> MERLVWDKLTLLGFLEKNHIPQKLYYNLSSQDKELSAEIQSNVTYYTLRDANNTLIQALIPISQDLQIHIYKKGEDYFLDFIPIIFTRKEKTLLLSLQTSPYQDIIKATNDPLLANQLMNAYKKSVPFKRLVKNDKIAIV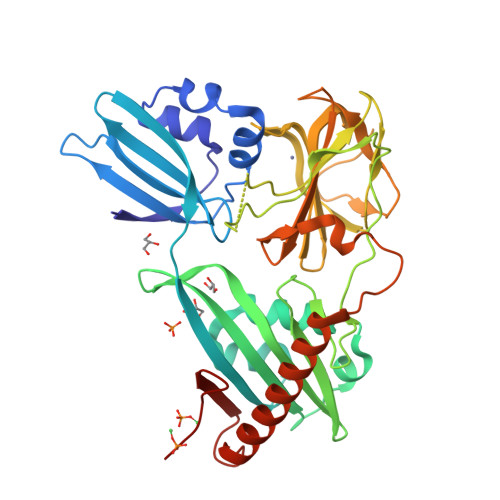YTRDYRVGQAFGQPTIKMAMVSSRSNQYYLFSHSNGHYYDSKAQEVAGFLLETPVKYTRISSPFSYGRFHPVLKVRRPHYGVDYAAKHGSLIHSASDGRVGFMGVKAGYGKVVEIHLNELRLVYAHMSAFANGLKKGSFVKKGQIIGRVGSTGLSTGPHLHFGVYKNSRPINPLGYIRTAKSKLHGKQREVFLEKAQRSKQKLEELLKTHSFEKNSFYLLEGFLEHHHHHH> EWTDSERFAITTL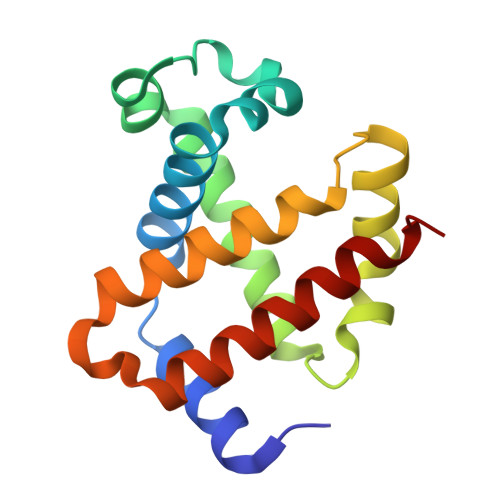WAKVNVESVGAQALVRLLVVYPWTQRYFGAFGNISDAAAIAGNAQVHAHGKTVLDSVGNAIAHMDDVADAFTALSTFHSETLHVDPDNFQHFGDCLSIVLAATFGTAYTPDVQAAWQKMIAVIISALSKEYH>[2x]CPRFLKVKNWETDVVLTDTLHLKSTLETGCTEHICMGSIVLPSQHTRKPEDVRTKDQLFP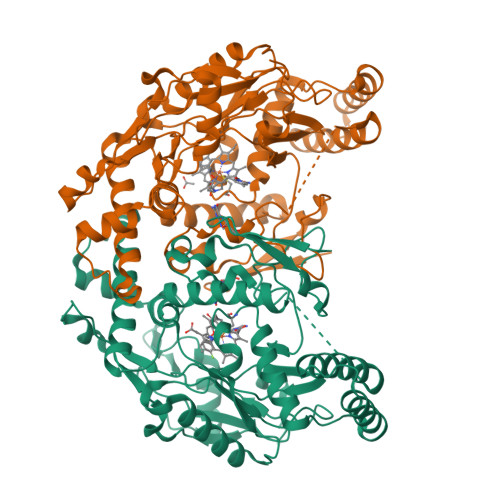LAKEFLDQYYSSIKRFGSKAHMDRLEEVNKEIESTSTYQLKDTELIYGAKHAWRNASRCVGRIQWSKLQVFDARDCTTAHGMFNYICNHVKYATNKGNLRSAITIFPQRTDGKHDFRVWNSQLIRYAGYKQPDGSTLGDPANVQFTEICIQQGWKAPRGRFDVLPLLLQANGNDPELFQIPPELVLEVPIRHPKFDWFKDLGLKWYGLPAVSNMLLEIGGLEFSACPFSGWYMGTEIGVRNYCDNSRYNILEEVAKKMDLDMRKTSSLWKDQALVEINIAVLYSFQSDKVTIVDHHSATESFIKHMENEYRCRGGCPADWVWIVPPMSGSITPVFHQEMLNYRLTPSFEAQPDPWNTHVWKG> MKYQQLEN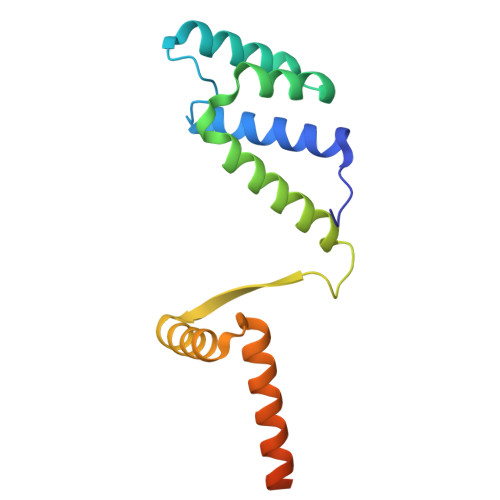LECGWKWAYLIRKHQEGEPITKYIENSAAHAAVDKLIKLESEPVRVLEWIEQHMNPDLFNRMKQTIRARRKRHFNAEHQHTRKKSIDLDFPVWHRLSALSQRRGNTLSETIVQLIEDAERKEKYANQMSSLKHDLEAILGKNE>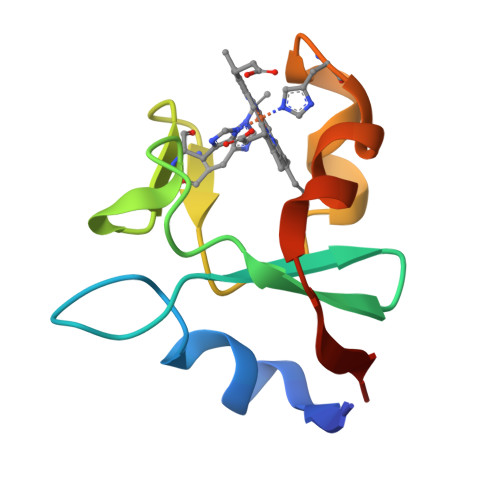 SMRVFTKEELSRYNGKEGAPAYVAYNGKVYDVTGSFHWKGGKHHVLHDAGQDLTESIGRAPHTAELLEKFPVVGVLRG High pressure atmospheres of argon and krypton were used to produce noble gas derivatives of crystals of three well studied MPs (two different proton pumps and a sodium light-driven ion pump). The structures obtained using X-ray crystallography showed that the vast majority of argon and krypton binding sites were located on the outer hydrophobic surface of the MPs – a surface usually accommodating hydrophobic chains of annular lipids (which are known structural and functional determinants for MPs). Taken together, the results obtained show that, in addition to binding in internal cavities within the MPs, noble gas atoms interact with MP hydrophobic surface at many sites and displace lipid molecules bound to their surfaces. In the experiments described here, we extend our knowledge as to how noble gas atoms bind to MP molecules, showing that they readily interact with the outer hydrophobic surface of MPs by non-specific binding at multiple sites and in particular compete with binding of lipids to the surfaces of the systems studied.

In total, 47, 35, 11 and 19 noble gas atoms were identified as partially occupying positions in the four crystal structures (tmBR-argon, tmBR-krypton, KR2-krypton, MAR-krypton, respectively). A good consistency is observed between argon and krypton binding positions: of 35 noble gas atom positions identified in tmBR-krypton, only two—which have low occupancy (0.1)—do not match corresponding sites in tmBR-argon. Moreover, at many positions (11, 13, 8 and 6, for tmBR-argon, tmBR-krypton, MAR-krypton and KR2-krypton, respectively), noble gas atoms replaced, at least partially, lipid atoms, with an altered conformation of lipid chains being sometimes clearly visible. Native datasets were also collected from crystals of the same batch for tmBR and MAR at ambient pressure. Overall, the derivatised structures do not differ significantly from the native ones with Cα r.m.s.d. value not exceeding 0.3 Å; rare side chain position alteration was observed. For all the investigated protein systems, we observed slight decrease in dynamics in presence of a noble gas. This effect was more prominent for both tmBR structures, in the presence of argon and krypton. Inspection of the correspondence between noble gas positions in the crystallographic models and the MD simulations shows that almost all noble gas atoms positions observed in the former have a nearby counterpart peak in the latter.

> MQAQITGRPEWIWLALGAALMGLGALYFLVKGMGVSDPDAKKFYAITALVPAIAFTMYLSMLLGYGLTMVPFGGEQNPIYWARYADWLFTTPLLLLDLALLVDADQGTILALVGADGIMIGTGLVGALTKVYSYRFVWWAISTAAMLYILYVLFFGFTSKAESMRPEVASTFKVLRNVTVVLWSAYPVVWLIGSEGAGIVPLNIETLLFMVLDVSAKVGFGLILLRSRAIFGEAEAPEPSAGDGAAATSDGSGIEGRSGAPHHHHHHHH> MRIDIVTIFPACLDPLRQSLPGKAIESGLVDLNVHDLRRWTHDVHHSVDDAPYGGGPGMVMKAPVWGEALDEI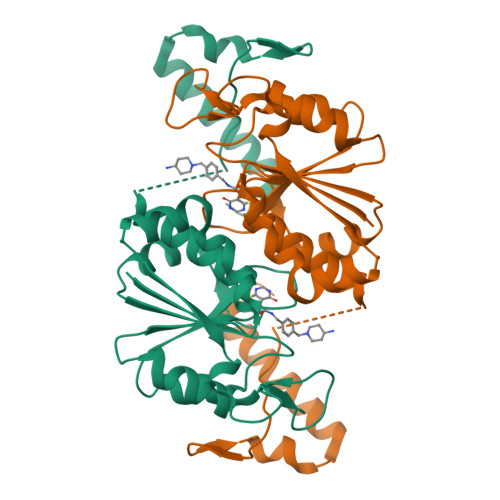CSSETLLIVPTPAGVLFTQATAQRWTTESHLVFACGRYEGIDQRVVQDAARRMRVEEVSIGDYVLPGGESAAVVMVEAVLRLLAGVLGNPASHQDDSHSTGLDGLLEGPSYTRPASWRGLDVPEVLLSGDHARIAAWRREVSLQRTRERRPDLSHPDGSHHHHHH> VRPLNCIVAVSQNMGIGKNGDLPWPPLRNEFKYFQRMTTTSSVEGKQNLVIMGRKTWFSIPEKNRPLKDRINIVLSRELKEPPRGAHFLAKSLDDALRLIEQPELASKVD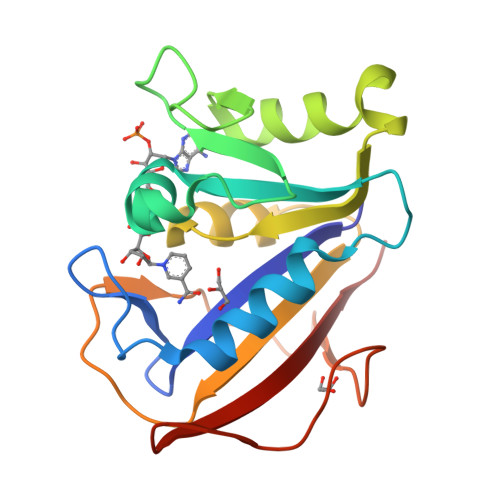MVWIVGGSSVYQEAMNQPGHLRLFVTRIMQEFESDTFFPEIDLGKYKLLPEYPGVLSEVQEEKGIKYKFEVYEKKD>ETGRTEAAPAAGQPVESFPLDFTAVEGNMDSFMAQVKSLAQSLYPCSAQQLNEDLRLHLLLNTSVTCNDGSPAGYYLKESRGSRRWLLFLEGGWYCFNRENCDSRYDTMRRLMSSRDWPRTRTGTGILSSQPEENPYWWNANMVFIPYCSSDVWSGASSKSEKNEYAFMGALIIQEVVRELLGRGLSGAKVLLLAGSSAGGTGVLLNVDRVAEQLEKLGYPAIQVRGLADSGWFLDNKQYRHTDCVDTITCAPTEAIRRGIRYWNGVVPERCRRQFQEGEEWNCFFGYKVYPT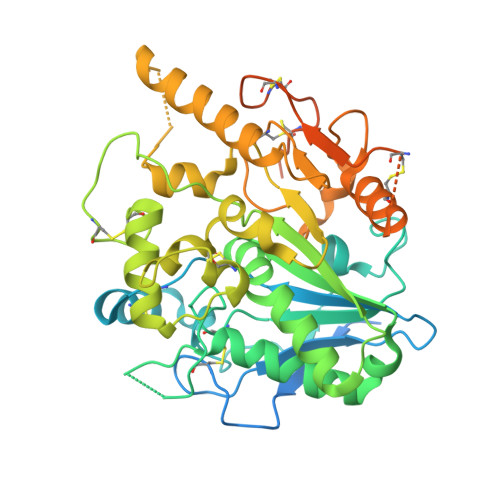LRCPVFVVQWLFDEAQLTVDNVHLTGQPVQEGLRLYIQNLGRELRHTLKDVPASFAPACLSHEIIIRSHWTDVQVKGTSLPRALHCWDRSLHDSHKASKTPLKGCPVHLVDSCPWPHCNPSCPTVRDQFTGQEMNVAQFLMHMGFDMQTVAQPQGLEPSELLGMLSNGSGTKHHHHHH[4x];> AAAAAAAAAA> MTGGMKPPARKPRILNSDGSSNITRLGLEKRGWLDDHYHDLLTVSWPVFITLITGLYLVTNALFALAYLACGDVIENARPGSFTDAFFFSVQTMATIGYGKLIPIGPLANTLVTLEALCGMLGLAVAASLIYARFTRPTAGVLFSSRMVISDFEGKPTLMMRLANLRIEQIIEADVHLVLVRSEISQEGMVFRRFHDLTLTRSRSPIFSLSWTVMHPIDHHSPIYGETDETLRNSHSEFLVLFTGHHEAFAQNVHARHAYSCDEIIWGGHFVDVFTT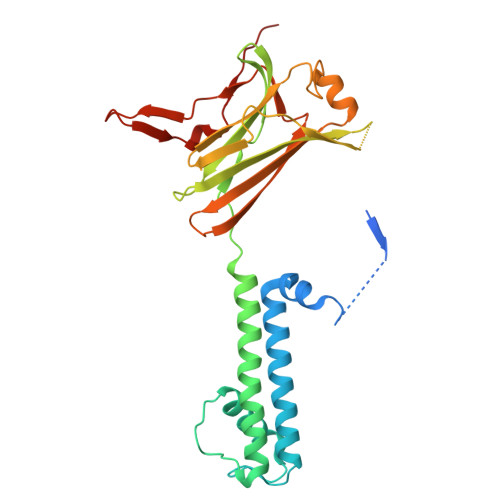LPDGRRALDLGKFHEIAQHHHHHH4-fluorooxepine-2,7-dione | C6 H3 F O3 | 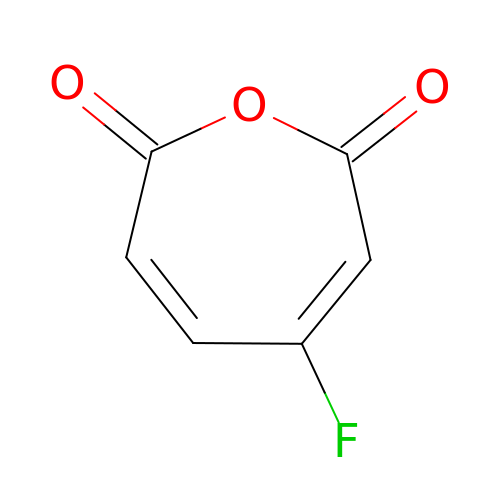MARYQJLDFKFFCO-UHFFFAOYSA-N>[8x]GVTFDDGAYTGIREINFEYNSETAIGGLRVTYDLNGMPFVAEDHKSFITGFKPVKISLEFPSEYIV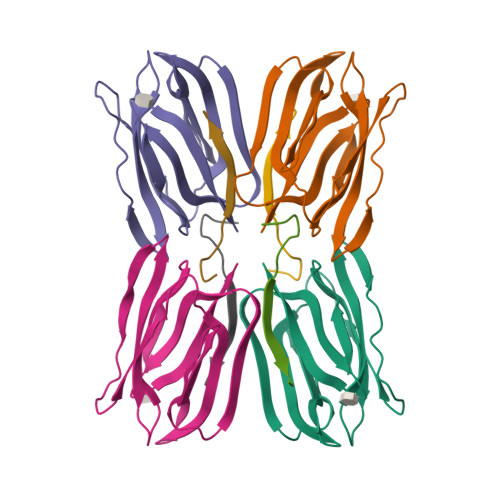EVSGYVGKVEGYTVIRSLTFKTNKQTYGPYGVTNGTPFSLPIENGLIVGFKGSIGYWLDYFSIYLSL;>[8x]RNGKSQSIIVGPWGD>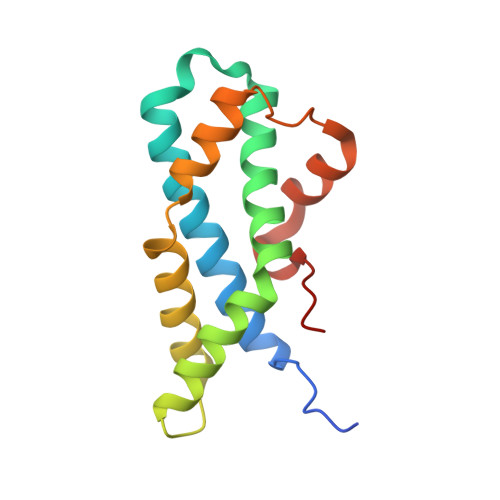MGRSWHYVEPKFLNKAFEVALKVQIIAGFDRGLVKWLRVHGRTLSTVQKKALYFVNRRYMQTHWANYMLWINKKIDALGRTPVVGDYTRLGAEIGRRIDMAYFYDFLKDKNMIPKYLPYMEEINRMRPADVPVKYMGK[6x]>[2x]ASYGKKTQMSILEQRESLPIYKLKEQLVQAVHDNQILIVIGETGSGKTTQITQYLAEAGYTSRGKIGCTQPRRVAAMSVAKRVSEEFGCCLGQEVGYTIRFEDCTSPETVIKYMTDGMLLRECLIDPDLTQYAIIMLDEAHERTIHTDVLFGLLKKTVQKRQDMKLIVTSATLDAVKFSQYFYEAPIFTIPGRTYPVEILYTKEPETDYLDASLITVMQIHLTEPPGDILVFLTGQEEIDTACEIL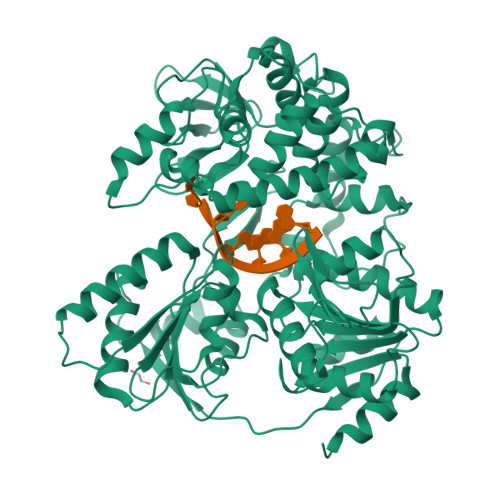YERMKSLGPDVPELIILPVYSALPSEMQTRIFDPAPPGSRKVVIATNIAETSLTIDGIYYVVDPGFVKQKVYNSKTGIDQLVVTPISQAQAKQRAGRAGRTGPGKCYRLYTERAYRDEMLTTNVPEIQRTNLASTVLSLKAMGINDLLSFDFMDAPPMETLITAMEQLYTLGALDDEGLLTRLGRRMAEFPLEPMLCKMLIMSVHLGCSEEMLTIVSMLSVQNVFYRPKDKQALADQKKAKFHQTEGDHLTLLAVYNSWKNNKFSNPWCYENFIQARSLRRAQDIRKQMLGIMDRHKLDVVSCGKSTVRVQKAICSGFFRNAAKKDPQEGYRTLIDQQVVYIHPSSALFNRQPEWVVYHELVLTTKEYMREVTTIDPRWLVEFAPAFFKVSDPTKLSKQKKQQRLEPLYNRYEEPNAWRISRAFRRR> MPHDPGATRLLAISPHLDDAVLSFGAGLAQAAQDGANVLVYTVFAGAAQPPYSPAAQRMHTIWGLAPDDDAVLYRRKEDIAALDHLRVAHRHGRFLD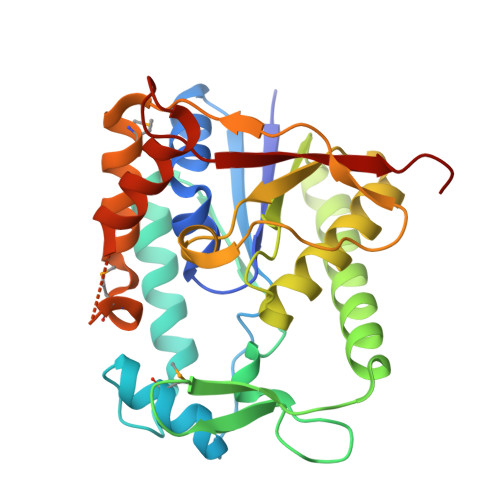SIYRKLPDGRWLTAHVEGRQKLAVNDHSPDSDHDLVGEVADDIRSIIDEFDPTLVVTCAAIGEHPDNEATRDAALFATHEKNVPVRLWEDLPYAVFKSGAVELPQGFRLGSADVSSVKPEMRSQKFQAVERYSSQMVLLNGSENNLFDRLDEHARQNAPHGGYGETTWPVVRSDDS>[8x]MTWLPLNPIPLKDRVSMIFLQYGQIDVIDGAFVLIDKTGIRTHIPVGSVACIMLEPGTRVSHAAVRLAAQVGTLLVWVGEAGVRVYASGQPGGARSDKLLYQAKLALDEDLRLKVVRKMFELRFGEPAPARRSVEQLRGIEGSRVRATYALLAKQYGVTWNGRRYDPKDWEKGDTINQCISAATSCLYGVTEAAILAAGYAPAIGFVHTGKPLSFVYDIADIIKFDTVVPKAFEIARRNPGEPDREV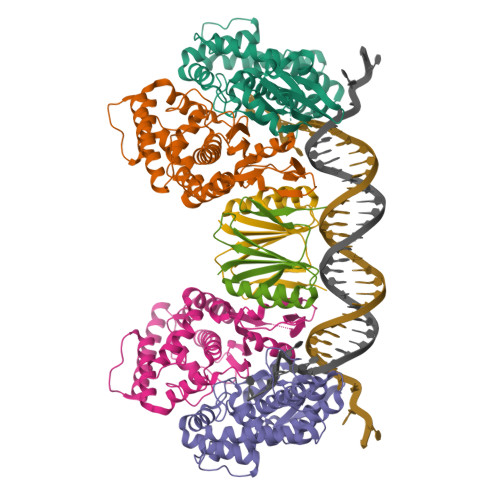RLACRDIFRSSKTLAKLIPLIEDVLAAGEIQPPAPPEDAQPVAIPLPVSLGDAGHRSS;>[4x]MSMLVVVTENVPPRLRGRLAIWLLEVRAGVYVGDVSAKIREMIWEQIAGLAEEGNVVMAWATNTETGFEFQTFGLNRRTPVDLDGLRLVSFLPV>KKLINSQISLLIGKGLHEFDSLRDPEVNDFRTKMRQFCEEAAAHRQQLGWVEWLQYSFPLQLEPSARGWRAGLLRVSNRALLVNVKFEGSEESFTFQVSTKDMPLALMACALRKKATVFRQPLVEQPEEYALQVNGRHEYLYGNYPLCHFQYICSCLHSGLTPHLTMVHSSSILAMRDEQSNPAPQVQKPRAKPPPIPAKKPSSVSLWSLEQPFSIELIEGRKVNADERMKLVVQAGLFHGNEMLCKTVSSSEVNVCSEPVWKQRLEFDISVCDLPRMARLCFALYAVVEKAKKARSTKKKSKKADCPIAWANLMLFDYKDQLKTGERCLYMWPSVPDEKGELLNPAGTVRGNPNTESAAALVIYLPEVAPHPVYFPALEKILELGRHGERGRITEEELQLREILERRGSGELYEHEKDLVWKMRHEVQEHFPEALARLLLVTKWNKHEDVAQMLYLLCSWPELPVLSALELLDFSFPDCYVGSFAIKSLRKLTDDELFQYLLQLVQVLKYESYLDCELTKFLLGRALANRKIGHFLFWHLRSEMHVPSVALRFGLIMEAYCRGSTHHMKVLMKQGEALSKLKALNDFVKVSSQKTTKPQTKEMMHMCMRQETYMEALSHLQSPLDPSTLLEEVCVEQCTFMDSKMKPLWIMYSSEEAGSAGNVGIIFKNGDDLRQDMLTLQMIQLMDVLWKQEGLDLRMTPYGCLPTGD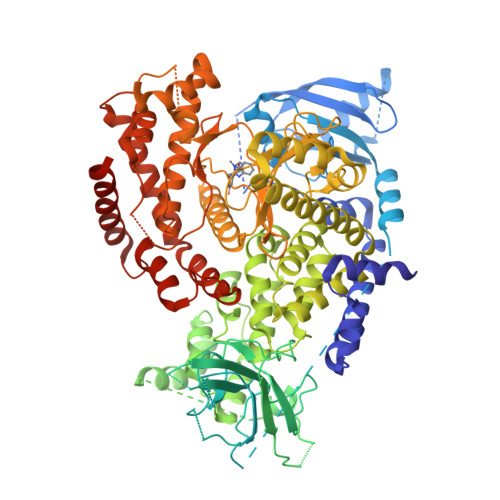RTGLIEVVLHSDTIANIQLNKSNMAATAAFNKDALLNWLKSKNPGEALDRAIEEFTLSCAGYCVATYVLGIGDRHSDNIMIRESGQLFHIDFGHFLGNFKTKFGINRERVPFILTYDFVHVIQQGKTNNSEKFERFRGYCERAYTILRRHGLLFLHLFALMRAAGLPELSCSKDIQYLKDSLALGKTEEEALKHFRVKFNEALRESWKTKVNWLAHNVSKDNRQ[2x]>MVDITGNGMAATAPTDERIVDKPLPQPQIRSGNVRAMPAARKLAQEHGIDLSTLTGSGPGGVIVKEDVERAITARAVPVSPLQRVNFYSAGYRLDGLLYTPRHLPAGERRPGVVLLVGYTYLKTMVMPDIAKVLNAAGYVALVFDYRGFGESEGPRGRLIPLEQVADARAALTFLAEQSMVDPDRLAVIGISLGGAHAITTAALDQRVRAVVALEPPGHGARWLRSLRRHWEWRQFLSRLAE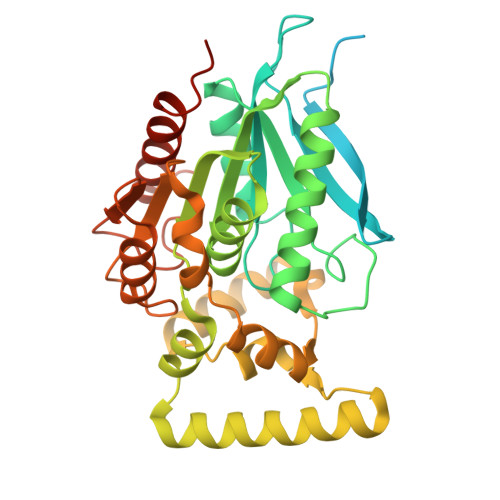DRRQRVLSGGSTMVDPLEIVLPDPESQAFLDQVAAEFPQMKVTLPLESAEALIEYVSEDLAGRIAPRPLLIIHSDADQLVPVAEAQAIAERAGSSAQLEIIPGMSHFNWVMPGSPGFTRVTDSIVKFLRNTLPVSADNLEHHHHHH[2x]>[5x]MRGSHHHHHHGSECGPALFQSDMTFKIFIDGEVNGQKFTIVADGSSKFPHGDFNVHAVCETG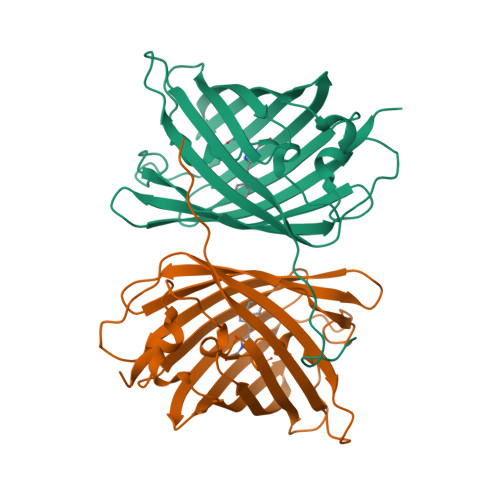KLPMSWKPICHLIQWGEPFFARYPDGISHFAQECFPEGLSIDRTVRFENDGTMTSHHTYELSDTCVVSRITVNCDGFQPDGPIMRDQLVDILPSETHMFPHGPNAVRQLAFIGFTTADGGLMMGHLDSKMTFNGSRAIEIPGPHFVTIITKQMRDTSDKRDHVCQREVAHAHSVPRITSAIGSDQD>[4x]MNKEVIPVTEIPKFQSRAEEFFPIQWYKEMLNNSPVYFHEETNTWNVFQYEHVKQVLSDYEFFSSDGQRTTIFVGDNSKKKSTSPITNLTNLDPPDHRKARSLLAAAFTHRSL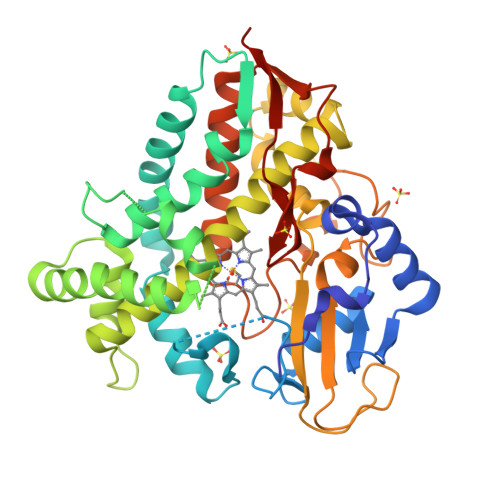KNWEPRIKQIAADLVEAIQKNPTINIVDDLSSPFPSLVIADLFGVPVKDRYQFKKWVDILFQPYDQERLEEIEQEKQRAGAEYFQYLYPIVIEKRSNLSDDIISDLIQAEFDGETFTDEEIVHATMLLLGAGVETTSHAIANMFYSFLYDDKSLYSELRNNRELAPKAVEEMLRYRFHISRRDRTVKQDNELLGVKLKKGDVVIAWMSACNMDETMFENPFSVDIHRPTNKKHLTFGNGPHFCLGAPLARLEMKIILEAFLEAFSHIEPFEDFELEPHLTASATGQSLTYLPMTVYRHHHHHH> IAAILVANAKEPCPPENLQLTPRALVGKWYLRTTSPDIFKQVSNITEFYSAHGNDYYGTVTDYSPEYGLEAHRVNLTVSGRTLKFYMNDTHEYDSEYEILA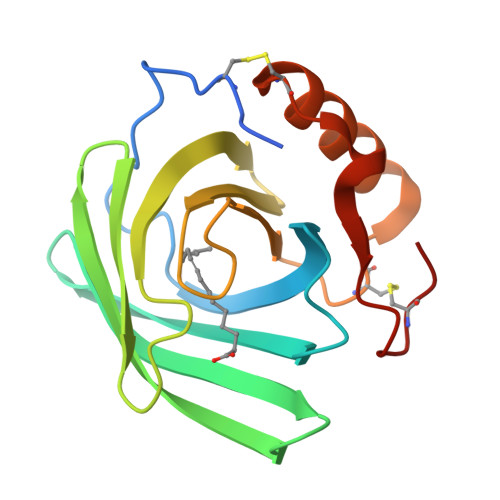VDKDYFIFYGHPPAAPSGLALIHYRQSCPKEDIIKRVKKSLKNVCLDYKYFGNDTSVHCRYLE>[4x]GMNLLLSDDYLLQDYPENITNTIRSGHSTCVRFNRKGDFLASGRVDGTVVIWDLETMGVARKLRGHSKNITSLSWSRCGRYLLSACQGWKVILWDLQDGKRYREVRFRAPVYGAELHPWNHHQFAAALFEDQPMLVDITEPVEVRYVLPSVPKRTSTETDPALREKQAKEDAKHMTTAIVYTASGDHLLAGT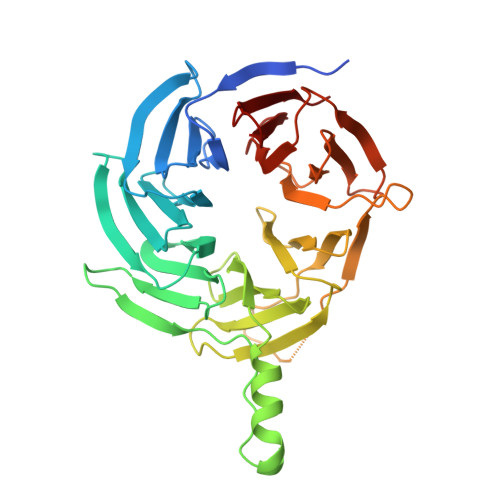TKGRLNIIDARTREIIYSEKIASGIITTLRLTESGRELLVNAQDRIIRTFIVPNLSAADLDPDTIQLPLEHKFQDVVNRLSWNHVAFSATGEYVAASTYNNHELYIWERGHGSLVRMLEGPKEEQGVIEWHPHRALLAACGLETGRINIWSVT In contrast, bacteria utilise the FASII system which involves a series of discrete and functionally specific enzymes that produce fatty acids primarily destined for incorporation into membrane lipids. FabG (3-oxoacyl-ACP or β-ketoacyl-ACP reductase) converts β-ketoacyl-ACP to β-hydroxyacyl-ACP in the presence of NADH or NADPH. FabG enzymes belong to the vast superfamily of SDRs that play a broad number of biological roles in eukaryotes, prokaryotes, and archaea, typically sharing 15–30% sequence identity and ‘fingerprint’ motifs. We provide high quality crystal structures for three enzymes: a functional low molecular weight FabG, a putative FabG protein, AbSDR, and a HMwFabG.

For FabG, the presence of a basic residue in the Gly motif (TGASRGIG18) suggested preference for NADPH and categorization into the cP1 subfamily. To observe binding mechanisms, we performed co-crystallization with NADPH. Crystals diffracted on the MX1 beamline at the Australian Synchrotron to a resolution of 1.85 Å in the spacegroup P 43 21 2 and the final model displayed good stereochemistry and an overall Rwork and Rfree of 0.16 and 0.19 respectively. The crystallographic asymmetric unit revealed two protomers, and strong positive density allowing NADPH to be modelled within each protomer. The NADPH is bound through an extensive binding pocket, whereby the nicotinamide moiety is bonded with Lys155 and Tyr151, and the adenine ribose is bonded through Ser14, Arg15, Thr37, Asp59, Val60, and Asn86. Interestingly, contrary to previous reports of large conformation changes in FabG upon coenzyme binding (such as that in E. coli), our structure reveals little change at the active site between apo and holo proteins (chain A comparison reveals r.m.s.d = 0.107 Å). Enzyme assays complemented clear preference for NADPH by FabG, confirming biological relevance for the NADPH bound structure. Overall, analysis of the FabG sequence, structure, and enzymatic assays, suggests FabG (ABO11256.2) is indeed a functional, and is likely the primary 3-oxoacyl-ACP reductase of A. baumannii.

>[2x]MTQERKVALVTGASRGIGAAIAQQLIQDGYFVVGTATSESGAQKLTDSFGEQGAGLALDVRNLDEIEAVVSHIEQNYGPVLVLVNNAGITKDNLLLRMSEDDWDDILNIHLKAVYRLSKRVLKGMTKARFGRIINISSVVAHFANPGQANYSAAKAGIEAFSRSLAKEMGSRQITVNSVAPGFIATEMTDALSEDIRKKMSDQVALNRLGEPQDIANAVSFLASDKAGYITGTVLHVNGGLYMA> GTSTQTKAGSLTIVGTGIESIGQMTLQALSYIEAAAKVFYCVIDPATEAFILTKNKNCVDLYQYYDNGKSRLNTYTQMSELMVREVRKGLDVVGVFYGHPGVFVNPSHRALAIAKSEGYRARMLPGVSAEDCLFADLCIDPSNPGCLTYEASDFLIRDRPVSIHSHLVLFQVGCVGIADFNFTGFDNNKFGVLVDRLEQEYGAEHPVVHYIAAMMPHQDPVTDKYTVAQLREPEIAKRVGGVSTFYIPPKARKASNLDIIRRLELLPAGQVPDKKARIYPANQWEPDVPEVEPYRPSDQAAIAQLADHAPPEQYQPLATSKAMSDVMTKLALDPKALADYKADHRAFAQSVPDLTPQERAALELGDSWAIRCAMKNMPSSLLDAARESGEEASQNGFPWVIVVGPIGVIGS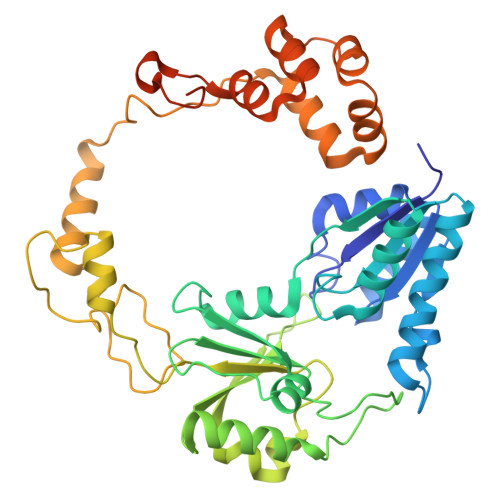VMSTE>AMMNALELQALRRIFDMTIEECTIYITQDNNSATWQRWEAGDIPISPEIIARLKEMKARRQRRINAIVDKINNRIGNNTMRYFPDLSSFQSIYTEGDFIEWKIYQSVAAELFAHDL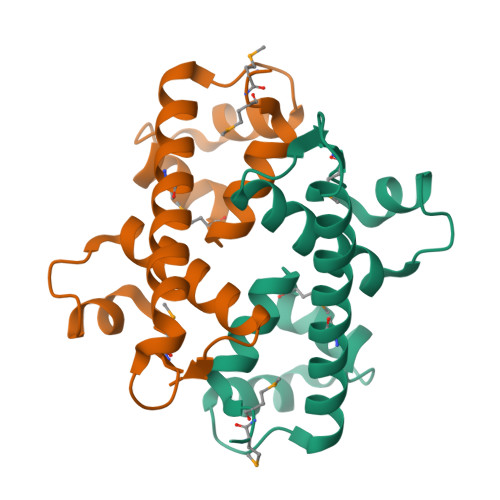ERLC[2x]>MGHHHHHHENLYFQGAPTEQRPGVQECYHGNGQSYRGTYSTTVTGRTCQAWSSMTPHSHSRTPEYYPNAGLIMNYCRNPDAVAAPYC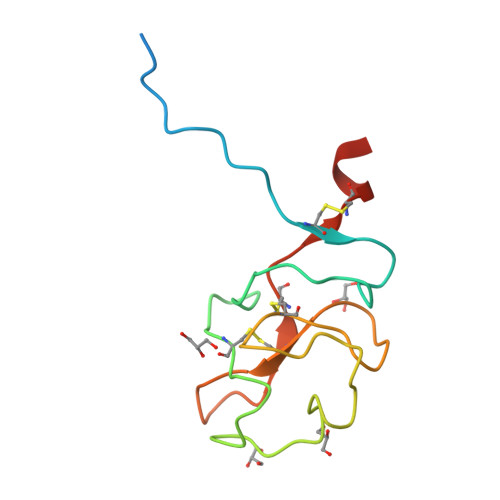YTRDPGVRWEYCNLTQCSDAEGTA[3x]> GHMDSFFRKKAIVRMSQNSLLDLYAHPTVVARFSEMAALHPHREAIRDRFGSVDYRQLLDSAEQLSDYLLEHYPQPGVCLGVYGEYSRESITCLLAILLSGHHYLYIDLKQPAAWNAELCRQVDCRLILDCSTTPTPANGLPCVPVRHLPAAPASVARPCFAADQIAYINFSSGTTGRPKAIACTHAGITRLCLGQSFLAFAPQMRFLVNSPLSFDAATLEIWGALLNGGCCVLNDLGPLDPGVLRQLIGERGADSAWLTASLFNTLVDLDPDCLGGLRQLLTGGDILSVPHVRRALLRHPRLHLVNGYGPTENTTFTCCHVVTDDDLEEDDIPIGKAIAGTAVLLLDEHGQEIAEPDRAGEIVAFGAGLAQGYRNDAARTRASFVELPYRGRLLRAYRTGDRARYDEQGRLRFIGRGDGQVKLNGYRLDLPALEQRFRRQPGILDCALLVRERNGVKQLLCAWTGKADASPQALLRQLPTWQRPHACVRVEALPLTAHGKLDRAALLRRLEEPLERCASALDPDQRGCAQLWSELLGCEVGAADQDFFLCGGNSLLALQLVALCQSAGAGANLGLADLQAN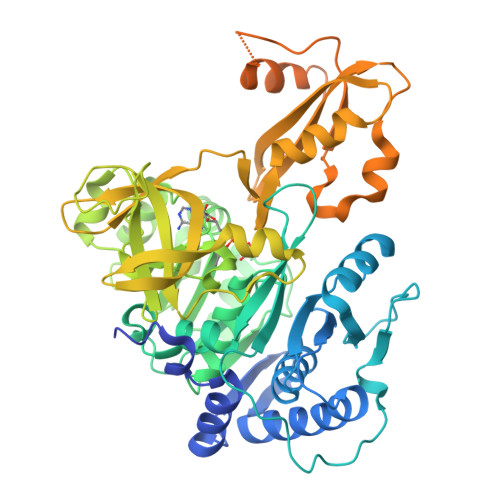SRLDQFSRLLRSHGLAPERLLERAATPEQPLVLSRSAA>[2x]SHMVNMVSNPGFEDGLDSWQDWQQDMSAVPEAAHNGALGLKIGGGKAAGGGQDIPLKPNTTYILGAWAKFDSKP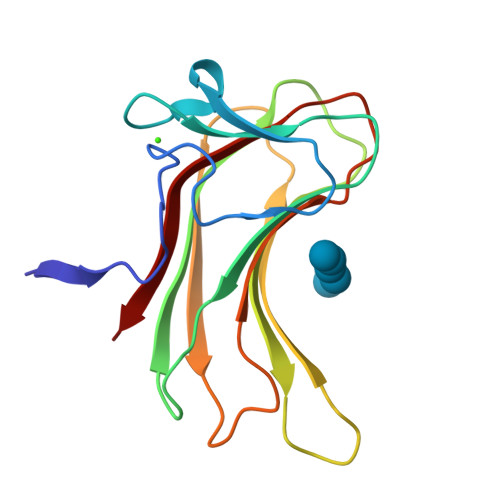AGTFDVVVQYHLKDANNTYVQHILNFNETDWTYKQLLFTTPDVFGSTPELALWKGDTSKANLYVDDVYLVEV>MRSRRVDVMDVMNRLILAMDLMNRDDALRVTGEVREYIDTVKIGYPLVLSEGMDIIAEFRKRFGCRIIANFKVADIPETNEKICRATFKAGADAIIVHGFPGADSVRACLNVAEEMGREVFLLTEMSHPGAEMFIQGAADEIA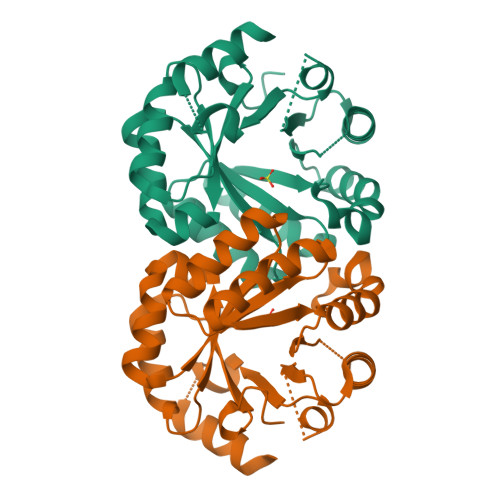RMGVDLGVKNYVGPSTRPERLSRLREIIGQDSFLISPGVGAQGGDPGETLRFADAIIVGRSIYLADNPAAAAAGIIESIKDLLNP[2x]> ELGKIDEYIECFYGETSVEKNKGAVALYELSKNPQNLTQLVNNETLMMALARVFREDWKKHFEVGTNIMNLFVNISKFSCLHGILLHHKIGTLCVNAMEHETKRYDFWIAEMKKTDQETLRKLKTAIRKQAMLLAACVTFLTNLATDISVELKMVRRNLVALLVKCLQMSSESTSSLTTATIKFLLKLSIFDENKIVMEQNGTIEKLLKLFPIQDPELRKAVIMLLFNFSFDSKNLPKMVNGGLVPHMASLLDSDTKALNMMYLLSCNDDAKAMLAYTDAIKLLMKDVLSGTGSEVTKAVLLNICLEKRNAQLVCGQRGQGLDLLMEMSINSRDLMLIKVVRAISSHEGATQNMFLKWIETLIGIAKNEGADNSESKSSFGLECMGTVAELKVAPWAKIIQSENLVPWMKTQLQEGIDESEEVTVLRDIKPLQLQIVIACGTMARQLDAARLLAPLIDTFVQLLQSCQIDDEFVVQLLYVFLQFLKHKELSARLMTQDSALGAHMIDLMHDANAVVREVCDNALLIMGEHSKEWAKRIAGERFKWHNAQWLEMVERDDSEFVDYDDEDFGAD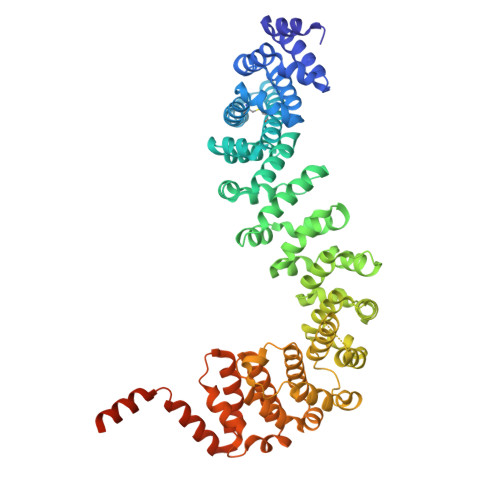LKFDHYDDGFDMNEPLF> ELPIARRASLHRFL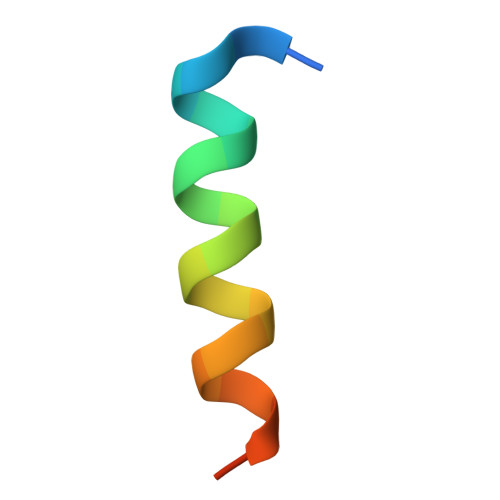EKRKDRVT> EEQEMFRDFDY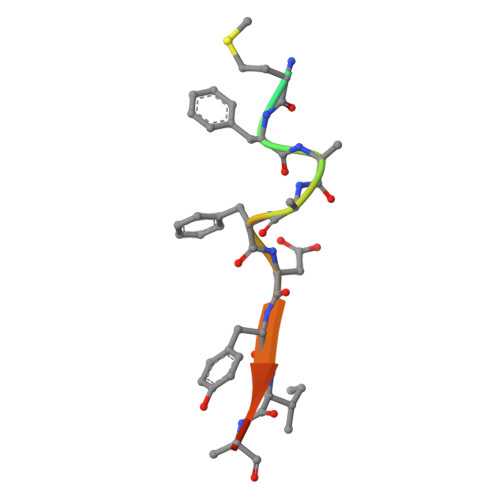IADW> GILRPRERLLLNALKKEADIRYRGRRMHKRFRSWAQQRVRHYWLPQKVCVTSDPQLMDGSYIAACVQKAATLRKHDLQLWHGFSKRILELADSLTPQQMGYIFYGYGKSLFRHEELYRGLLPFVAEALPEFHSHALMTVAWALERVRVNDRAVVAQIAEEALAKKDLMRPADFIKIVNC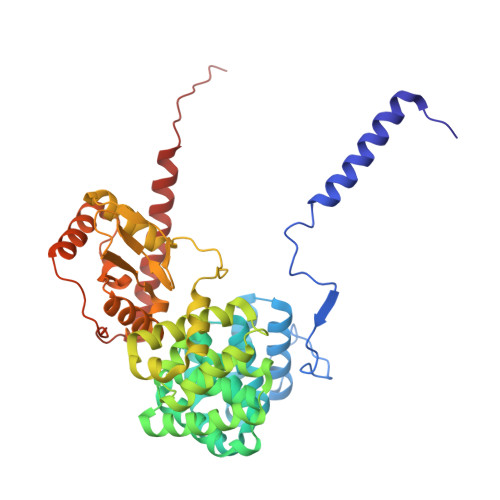VARMGAAPPSLAAALSAELMRVLDEKCNALLFRGAVDHVAVATLYSDPLRLYLLERFTKTAICCRPMHYQKAFQSAVAIRVLHPPVWQQLSKAVRNFYIRLSLRRIPQRARRPSPLHWDVSNALAKLGVFHRNTFQWGCFWIDIGEIDDRRQCWFVDGPSDFYSSTNEYTEANKLQHRILSELGWNIRRVRWNDWVQLGTDMDAKVEYLRKLRERPPWPAILTDGPSSSRQEMVANLRSARDVQRALKERREKNRQPHSLVMNL> GHMVKSGLQIKKNAIIDDYKVTSQVLGLGINGKVLQIFNKRTQEKFALKMLQDCPKARREVELHWRASQCPHIVRIVDVYENLYAGRKCLLIVMECLDGGELFSRIQDRGDQAFTEREASEIMKSIGEAIQYLHSINIAHRDVKPENLLYTSKRPNAILKLTDFGFAKETTGHNSLTTPCYTPYYVAPEVLGPEKYDKSCDMWSLGVIMYILLCGYPPFYSNHGLAISPGMKTRIRMGQYEFPNPEWSEVSEEVKMLIRNLLKTEPTQRMTITEFMNHPWIMQSTKVPQTPLHTSRVLKEDKERWEDVKEEMTSALAT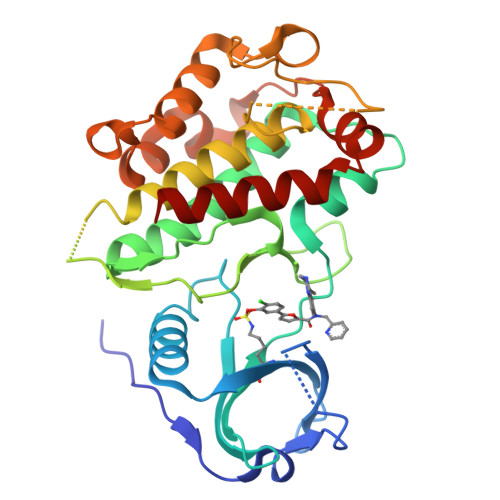MR> KLSEHLRYCDSILREMLSKKHAAYAWPFYKPVDAEALELHDYHDIIKHPMDLS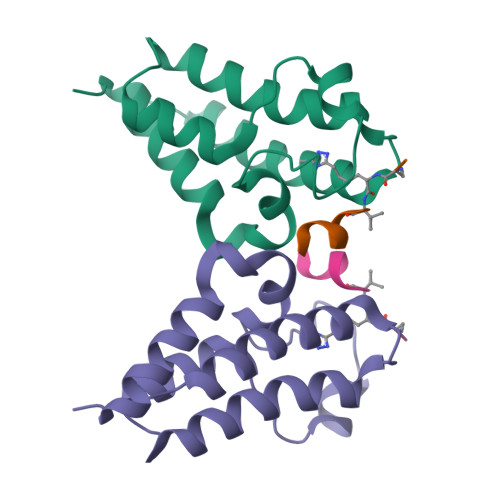TVKRKMDGREYPDAQGFAADVRLMFSNCYKYNPPDHEVVAMARKLQDVFEMRFAKMP;> HRXVLRDNY> MGSSHHHHHHSQDLMVTSTYIPMSQRRSWADVKPIMQDDGPNPVVPIMYSEEYKDAMDYFRAIAAKEEKSERALELTEIIVRMNPAHYTVWQYRFSLLTSLNKSLEDELRLMNEFAVQNLKSYQVWHHRLLLLDRISPQDPVSEIEYIHGSLLPDPKNYHTWAYLHWLYSHFSTLGRISEAQWGSELDWCNEMLRVDGRNNSAWGWRWYLRVSRPGAETSSRSLQDELIYILKSIHLIPHNVSAWNYLRGFLKHFSLPLVPILP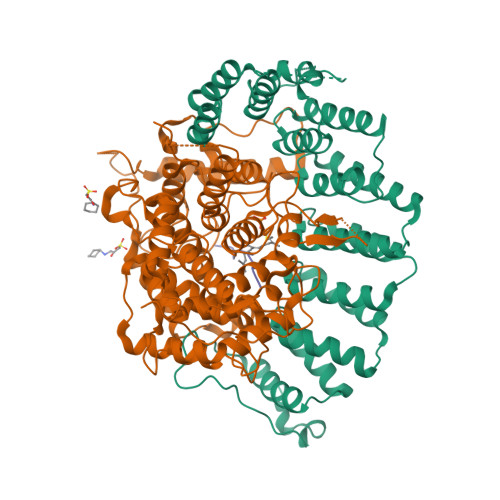AILPYTASKLNPDIETVEAFGFPMPSDPLPEDTPLPVPLALEYLADSFIEQNRVDDAAKVFEKLSSEYDQMRAGYWEFRRRECAE;> MATEFTPSVYSLVSKPLPSNSRPSATLDEQAETEDLISQLFDLTADPNALVSEHGKRYSGLRKQEHTQFLASSFFQLPGKFVSLDASRPWLVFWTVHSLDLLGVALDQGTKDRVVSTLLHFLSPKGGFGGGPANSQIPHLLPTYASVCSLAIAGNDSSTGGWKDLAAARQSIYEFFMRCKRPDGGFVVCEGGEVDVRGTYCLLVVATLLDIITPELLHNVDKFVSACQTYEGGFACASFPFPSVVPSTSAFPTSEPSCRVSMAEAHGGYTSCSLNSHFLLTSVPLPSFPLSIDANAALRWTVLQQGEPIEGGGFRGRTNKLVDGCYSWWVGGGAPVAEELVRREKSRKVKKSRIEVFEEEKEGDWEDVPPIPPIFNRVALQEFTLVAAQQDPGSTGGLRDKPGKRPDQYHTCNNLSGLSIAQHKMSHSPSTVSSNRLKFDASKGLPAVKPVAPGGGWKNEDERQNARREIWANALGWIEEEGGEIIVGGKDNRINTTTPVFNILGLRLKPFINYFYCQEN;> DDPTASACNIQ> MSTSNGSANGTNGVGLPRGDEPEIIAVRRGMFGNRDTGDTSGYGRLVRPV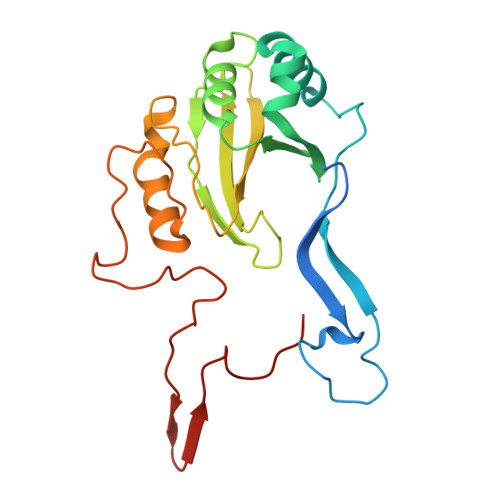ALPGSTPRPYGGYFDAVMDRLAEVLGEERYAMSIERVVVYRDQLTIEVSRVQLPAVASVLRDDPDLRFELCLGVSGVHYPEDTGRELHAVYPLMSITHNRRIQLEVAAPDADPHIPSLYAVYPTTDWHERETYDFFGIIFDGHPSLTRIEMPDDWEGHPQRKDYPLGGIPVEYHGAQIPPPDQRRSYS> MAPVIRRAKEIDLYCLNSLMYKLHDEHHQQCPDLFKTASEIEEEKSIARYLDDPECMVYVAEMDDVIIGFITGHFCELISTVSKLVMMATIDELYIEKEYRREGVAEQLMM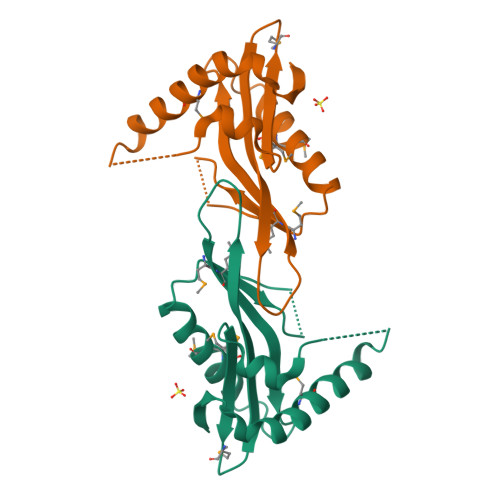RIEQELKDYGVKEIFVEVWDFNKGALEFYNKQGLNEHIHYLRKPLNRLEHHHHHH> GSSGSSGMIKEYRTIKEVVGPLMAVEKVSGVKYEELIEVRMQNGEIRRGQVLEVQEDKAMVQIFEGTSGICLKNSSVRFLGHPLQLGVSEDMIGRVFDGLGRPKDNGPEILPEKYLDINGEVINPIARDYPDEFIQTGISAIDHLNTLVRGQKLPVFSGSGLPHKELAAQIARQATVLDSSDDFAVVFAAIGITFEEAEFFMEDFRQTGAIDRSVMFMNLANDPAIERIATPRMALTAAEYLAYEKGMHVLVIMTDMTNYAEALREISAARREVPGRRGYPGYLYTNLATLFERAGRIRGLKGSVTQIPILTMPEDDKTHPIPDLTGYITEGQIILTRELYKSGIQPPIDVLPSLSRLKDKGTGAGKTREDHAATMNQLFAAYAQGKQAKELAVVLGESALSDIDKIYAKFAERFENEYVNQGFYTNRTITETLDLGWEL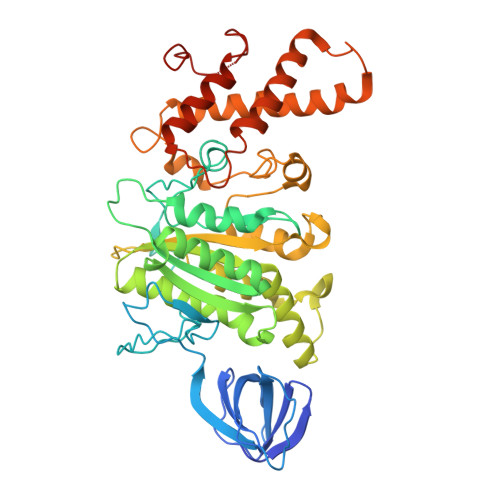LAMLPRTELKRIKDDLLDKYLPEGK(3S,5S,7aR)-5-(sulfanylmethyl)tetrahydro[1,3]thiazolo[4,3-b][1,3]thiazole-3-carboxylic acid | C7 H11 N O2 S3 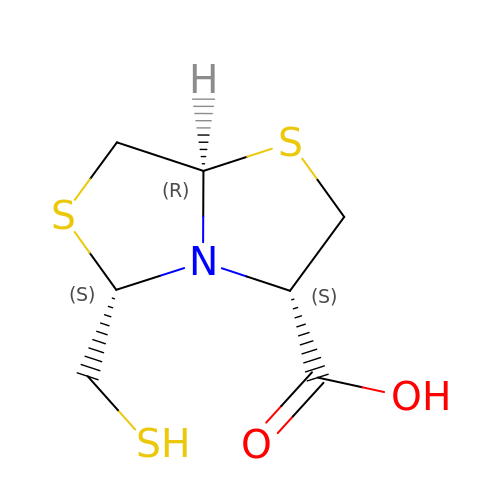| ZTWVMVSSSBGFHH-NGJCXOISSA-N>[7x]XXXXXXXXXXXXXXXXXXXXXXXXXXXXXXXXXXXXMIAELFTNNALNLVIIFGSCAALILMSFWFRRGNRKRKGFLFHAVQFLIYTIIISAVGSIINY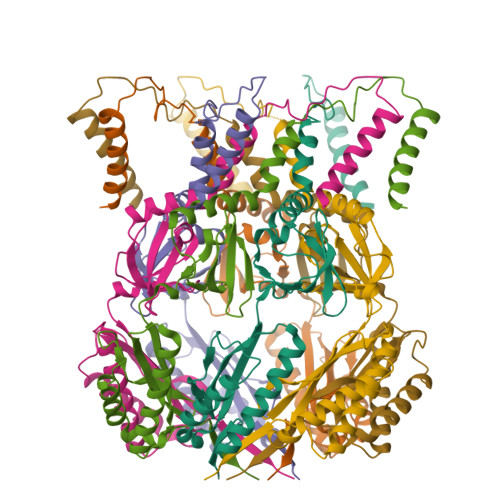VIENYKLKFITPGVIDFICTSLIAVILTIKLFLLINQFEKQQIKKGRDITSARIMSRIIKITIIVVLVLLYGEHFGMSLSGLLTFGGIGGLAVGMAGKDILSNFFSGIMLYFDRPFSIGDWIRSPDRNIEGTVAEIGWRITKITTFDNRPLYVPNSLFSSISVENPGRMTNRRITTTIGLRYEDAAKVGVIVEAVREMLKNHPAIDQRQTLLVYFNQFADSSLNIMVYCFTKTTVWAEWLAAQQDVYLKIIDIVQSHGADFAFPSQTLYMDNITPPEQGRLEHHHHHH> GGGGUUAUGUGUGCCCGGCAUGGGUGCAGUCUAUAGGGUGAGAGUCCCGAACUGUGAAGGCAGAAGUAACAGUUAGCCUAACGCAAGGGUGUCCGUGGCGACAUGGAAUCUGAAGGAAGCGGACGGCAAACCUUCGGUCUGAGGAACACGAACUUCAUAUGAGGCUAGGUAUCAAUGGAUGAGUUUGCAUAACAAAACAAAGUCCUUUCUGCCAAAGUUGGUACAGAGUAAAUGAAGCAGAUUGAUGAAGGGAAAGACUGCAUUCUUACCCGGGGAGGUCUGGAAACAGAAGUCAGCAGAAGUCAUA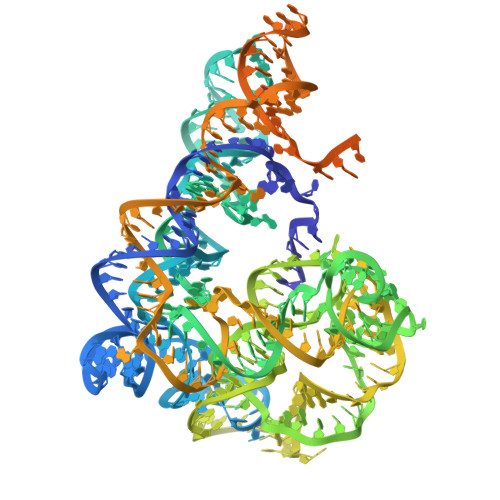GUACCCUGUUCGCAGGGGAAGGACGGAACAAGUAUGGCGUUCGCGCCUAAGCUUG> GSLIGLMKDAFQPHHHHHHHLSPHPPGTVDKKMVEKCWKLMDKVVRLCQNPKLALKNSPPYILDLLPDTYQHLRTILSRYEGKMETLGENEYFRVFMENLMKKTKQTISLFKEGKERMYEENSQPRRNLTKLSLIFSHMLAELKGIFPSGLFQGDTFRITKADAAEFWRKAFGEKTIVPWKSFRQALHEVHPISSGLEAMALKSTIDLTCNDYISVFEFDIFTRLFQPWSSLLRNWNSLAVTHPGYMAFLTYDEVKARLQKFIHKPGSYIFRLSCTRLGQWAIGYVTADGNILQTIPHNKPLFQALIDGFREGFYLFPDGRNQNPD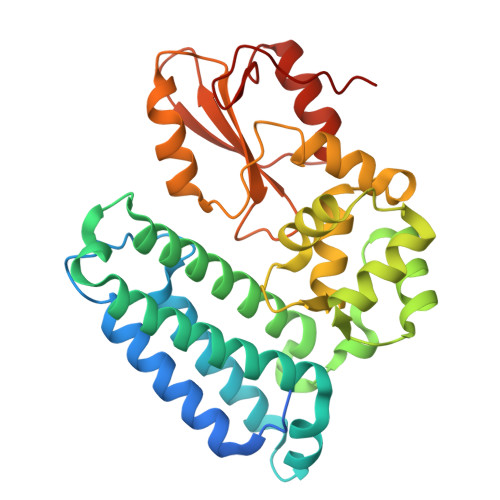LTG>MNKAELIDVLTQKLGSDRRQATAAVENVVDTIVRAVHKGDSVTITGFGVFEQRRRAARVARNPRTGETVKVKPTSVPAFRPGAQFKAVVSGAQRLPAEGPHHHHHH[2x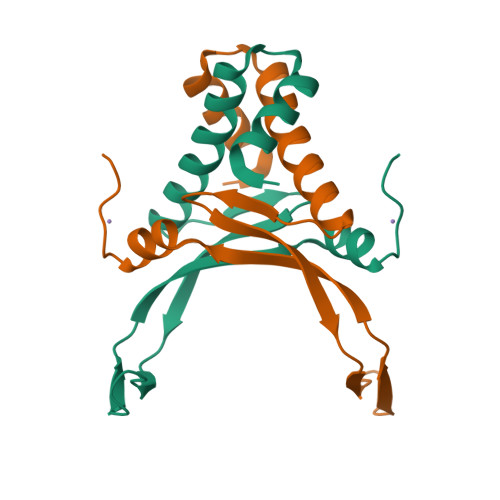]> MASSQKREGFAENGAKAVYDALKNDRNSYETRAENCAKYTIPSLFPKDSDNASTDYTTPWQAVGARGLNNLASKLMLALFPMQTWMKLTISEFEAKQLVAQ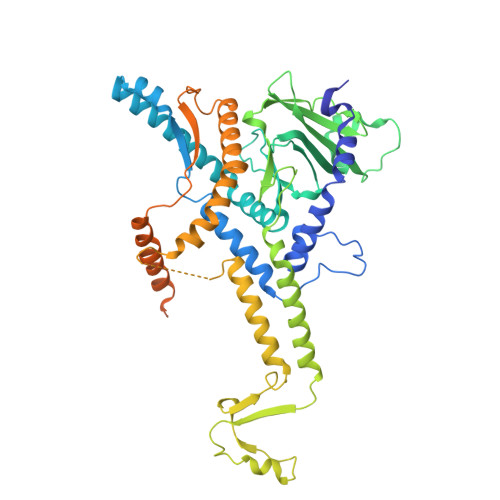PAELAKVEEGLSMVERILMNYIESNSYRVTLFETLKQLVVAGNALLYIPEPEGAYNPMKLYRLSSYVVQRDAFGTVLQIVTLDKTAYAALPEDVRNAMDSGQEHKGDEMIDVYTHIYLDEESGEYLKYEEIDGVEVDGTDASYPVDACPYIPVRMVRIDGESYGRSYCEEYLGDLRSLENLQEAIVKMSMISAKVIGLVNPAGITQVRRLTKAQTGDFVSGRPEDISFLQLEKAADFSVAKAVSEQIEGRLSYAFMLNSAVQRTGERVTAEEIRYVASELEDTLGGVYSILSQELQLPMVRVLLKQLQATNQIPELPKEAVEPTISTGMEALGRGQDLDKLERCIAAWSALAPMQNDPDINIATIKLRIANAIGIDTSGILKTPEEKQQEMAEAAQGTALENAAASAGAGAGALATASPENMEAAAAQAGMVPN>[2x]QRCGEQGSGMECPNNLCCSQYGYCGMG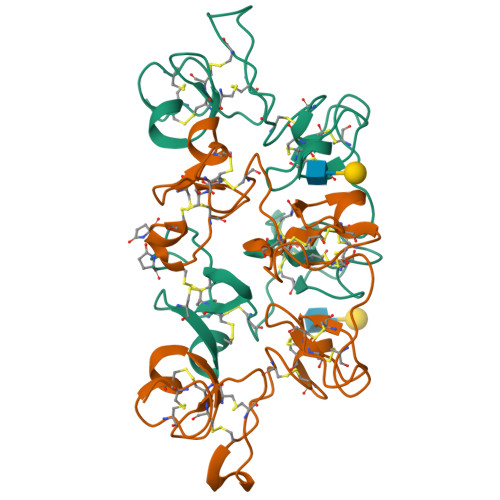GDYCGKGCQNGACWTSKRCGSQAGGKTCPNNHCCSQYGHCGFGAEYCGAGCQGGPCRADIKCGSQAGGKLCPNNLCCSQWGYCGLGSEFCGEGCQNGACSTDKPCGKDAGGRVCTNNYCCSKWGSCGIGPGYCGAGCQSGGCDGVFAEAIATNSTLLAE> MSIEPVFILVRPQMGENIGAAARAMLNFG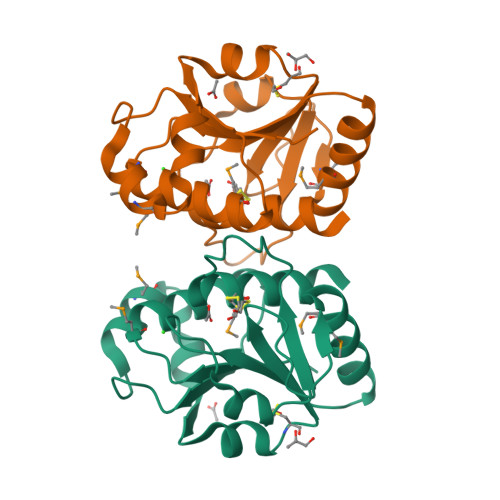LGRLRIVDPRDGWPNPKAVAMASGAGRLLDHAGLFPTVAEAIRDCDYVFATTARGRELTKPVMTPERAMAHGRALTGEGRRVGILFGPERTGLENEDVALANAIVTVPVNPEFFSLNLAQCVLLLAYEWRRQHDETPPEVIDMARVDFASGLEVEKLGDHFEEKLEAAGFFFPPEKAPGMKLNLRNMWARLPLTRADVQTLHGMLRQIAWKLKQENLYFQ>AKLMGQAMAKRVKATILYATETGKSQAYAKTLCEIFKHAFDAKAMSMEEYDIVHLEHEALVLVVTSTFGNGDPPENGEKFGCALMEMRHPNSVQEERKSYKVRFNSVSSYSDSRKSSGDGPDLRDNFESTGPLANVRFSVFGLGSRAYPHFCAFGHAVDTLLEELGGERILKMREGDELCGQEEAFRTWAKKVFKAACDVFCVGDDVNIEKPNNSLISNDRSWKRNKFRLTYVAEAPDLTQGLSNVHKKRVSAARLLSRQNLQSPKSSRSTIFVRLHTNGNQELQYQPGDHLGVFPGNHEDLVNALIERLEDAPPANHVVKVEMLEERNTALGVISNWKDESRLPPCTIFQAFKYYLDITTPPTPLQLQQFASLATNEKEKQRLLVLSKGLQEYEEWKWGKNPTMVEVLEEFPSIQMPATLLLTQLSLLQPRYYSISSSPDMYPDEVHLTVAIVSYHTRDGEGPVHHGVCSSWLNRIQADDVVPCFVRGAPSFHLPRNPQVPCILVGPGTGIAPFRSFWQQRQFDIQH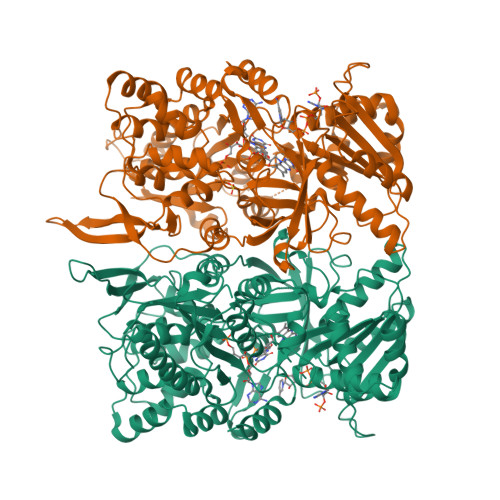KGMNPCPMVLVFGCRQSKIDHIYREETLQAKNKGVFRELYTAYSREPDRPKKYVQDVLQEQLAESVYRALKEQGGHIYVCGDVTMAADVLKAIQRIMTQQGKLSEEDAGVFISRLRDDNRYHEDIFGVTLRTYEVTNRLRSESIAFIEESKKDADEVFSS[2x]>GSNSLFGSVETWPWQVLSTGGKEDVSYEERACEGGKFATVEVTDKPVDEALREAMPKIMKYVGGTNDKGVGMGMTVPVSFAVFPNEDGSLQKKLKVWFRIPNQFQGSPPAPSDESVKIEEREGITVYSTQ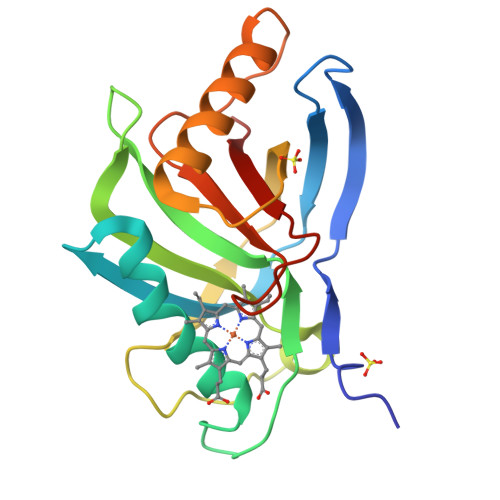FGGYAKEADYVAHATQLRTTLEGTPATYQGDVYYCAGYDPPMKPYGRRNEVWLVKA[2x]> MERNKLARQIIDTCLEMTRLGLNQGTAGLVSVRYQDGMLITPTGIPYEKLTESHIVFIDGNGKHEEGKLPASEWRFHMAAYQSRPDANAVVHNHAVHCTAVSILNRSIPAIHYMIAAAGGNSIPCAPYATFGTRELSEHVALALKNRKATLLQHHGLIACEVNLEKALWLAHEVEVLAQLYLTTLAITDPVP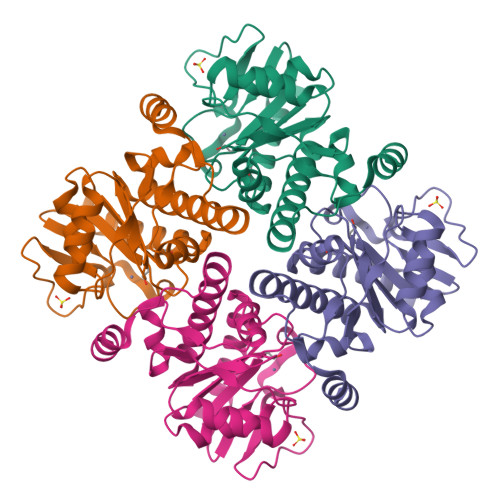VLSDEEIAVVLEKFKTYGLRIEE> EPLEADKCKEREEKIILVSSANEIDVRPCPLNPNEHKGTITWYK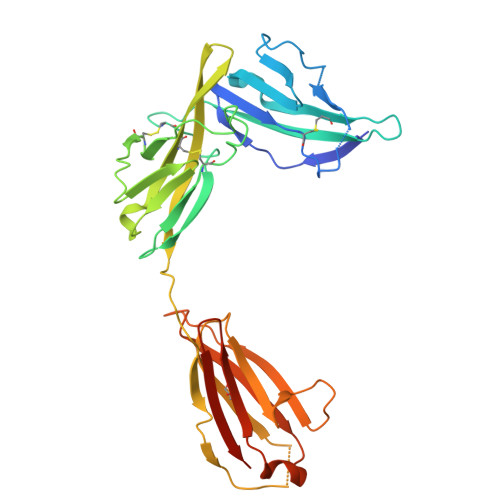DDSKTPVSTEQASRIHQHKEKLWFVPAKVEDSGHYYCVVRNSSYCLRIKISAKFVENEPNLCYNAQAIFKQKLPVAGDGGLVCPYMEFFKNENNELPKLQWYKDCKPLLLDNIHFSGVKDRLIVMNVAEKHRGNYTCHASYTYLGKQYPITRVIEFITLEENKPTRPVIVSPANETMEVDLGSQIQLICNVTGQLSDIAYWKWNGSVIDEDDPVLGEDYYSVENPANKRRSTLITVLNISEIESRFYKHPFTCFAKNTHGIDAAYIQLIYPVTNFQK>[2x]MASRGVNKVILVGNLGQDPEVRYMPSGGAVANLTLATSESWRDKQTGEMKEQTEWHRVVMFGKLAEVAGEYLRKGSQVYIEGQLRTRKWTDQSGQERYTTEINVPQIGGVMQMLGGHHHHHH

Single-stranded DNA (ssDNA)-binding proteins (SSBs) play a central role in cells by participating in DNA metabolism, including replication, repair, recombination, and replication fork restart. SSBs bind tightly and cooperatively to ssDNA, regardless of sequence, and prevent premature annealing and unwanted nuclease digestion. Most, but not all, bacterial SSBs are active as homotetramers, in which four oligonucleotide/oligosaccharide-binding (OB) folds form a DNA-binding domain. In this study, we determined the crystal structure and examined the size of the ssDNA-binding site of an SSB from Salmonella enterica serovar Typhimurium LT2 (SeSSB), a ubiquitous opportunistic pathogen which is highly resistant to antibiotics.

The SeSSB structure was determined at a resolution of 2.8 Å. Two monomers (subunit A and B) of the SeSSB were found in the asymmetric unit. Given that the oligomerization state of bacterial SSBs in solution is tetrameric, the crystallographically related tetramer A-B-A′-B′ is also shown. In both of the subunits, only the N-terminal ssDNA-binding domain (residues 1–115) was ordered and observed. Even in the N-terminal domain, residues in the loops L12 (residues 25–26) and L23 (residues 44–48) were disordered and unobserved. The core of the OB-fold in the SeSSB is made of a six-stranded β-barrel capped by an α-helix. The GGRQ motif, proposed as a regulatory switch for ssDNA binding, and the PXXP motifs, known to mediate the protein–protein interactions, were disordered and disappeared in our crystal structure. The corresponding residues in the SeSSB are W55, F61, and W89, which may play a similar role to that of EcSSB in ssDNA binding. Hydrogen bonds and salt bridges were formed at the dimer–dimer interface of the SeSSB: S3(A)–Q111(B′), G5(A)–Q111(B′), G5(B)–Q111(A′), Q111(A)–G5(B′), Q111(B)–S3(A′), and Q111(B)–G5(A′). The native molecular mass for SeSSB was approximately four times the mass of the monomer and therefore the SeSSB was a stable tetramer.>[3x]DDSLGEAVTTRAEALTIPAVLRARNLLSTTVARTPLVCDGTLPPFVPVAAPPGAATMQTPFHRMLATADDLLFNGVACWALDRDESGTCIGAIHIPLDTWQIEENTVRVNGKAVDPMEVCIFVGIHGGLLTHASETFTDARNLVRAAARVAQNPAALIELRQTNNAQLSPDDV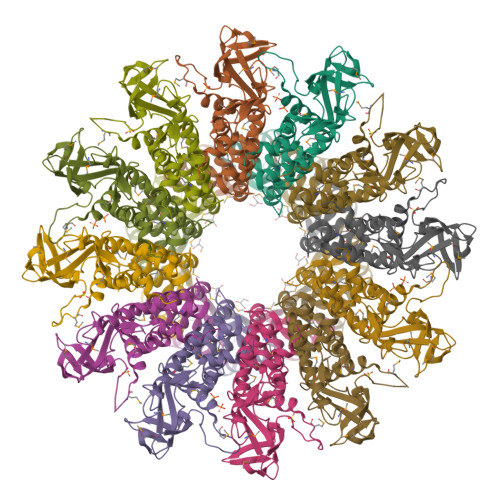DRIINGYVAARRGRNSGVGFSSSGLEVHEHEMAKENLLIEGRNAAAVDVARAMNVPAAFIDATVGGTSLSYQNAASRMIELVTFGVEPLMSAIEARLNQPDMHADHLANPLKFDPAALLDAIPTTPTIGAQPHGENS>MDDKELIEYFKSQMKEDPDMASAVAAIRTLLEFLKRDKGETIQGLRANLTSAIETLCGVDSSVAVSSGGELFLRFISLASLEYSDYSKCKKIMIERGELFLRRISLSRNKIADLCHTFIKDGATILTHAYSRVVLRVLEAAVAAKKRFSVYVTESQPDLSGKKMAKALCHLNVPVTVVLDAAVGYIMEKADLVIVGAEGVVENGGIINKIGTNQMAVCAKAQNKPFYVVAESFKFVRLFPLNQQDVPDKFKYKADTLKVAQTGQDLKEEHPWVDYTAPSLITLLFTDLGVLTPSAVSDELIKLYL[2x];>[2x]MPGSDYKDHDGDYKDHDIDYKDDDDKAAKGSELSERIESFVETLKRGGGPRSSEEMARETLGLLRQIITDHRWSNAGELMELIRREGRRMTAAQPSETTVGNMVRRVLKIIREEYGRLHGRSDESDQQESLHKLLTSGGLNEDFSFHYAQLQSNIIEAINELLVELEGTMENIAAQALEHIHSNEVIMTIGFSRTVEAFLKEAARKRKFHVIVAECAPFCQGHEMAVNLSKAGIETTVMTDAAIFAVMSRVNKVIIGTKTILANGALRAVTGTHTLALAAKHHSTPLIVCAPMFKLSPQFPNEEDSFHKFVAPEEVLPFTEGDILEKVSVHCPVFDYVPPELITLFISNIGGNAPSYIYRLMSELYHPDDHVL;>MEFQAVVMAVGGGSRMTDLTSSIPKPLLPVGNKPLIWYPLNLLERVGFEEVIVVTTRDVQKALCAEFKMKMKPDIVCIPDDADMGTADSLRYIYPKLKTDVLVLSCDLITDVALHEVVDLFRAYDASLAMLMRKGQDSIEPVPGQKGKKKAVEQRDFIGVDSTGKRLLFMANEADLDEELVIKGSILQKHPRIRFHTGLVDAHLYCLKKYIVDFLMENGSITSIRSELIPYLVRKQFSSASSQQGQEEKEEDLKKKELKSLDIYSFIKEANTLNLAPYDACWNACRGDRWEDLSRSQVRCYVHIMKEGLCSRVSTLGLYMEANRQVPKLLSALCPEEPPVHSSAQIVSKHLVGVDSLIGPETQIGEKSSIKRSVIGSSCLIKDRVTITNCLLMNSVTVEEGSNIQGSVICNNAVIEKGADIKDCLIGSGQRIEAKAKRVNEVIVGNDQLMEI[2x];>[2x]MAAVAVAVREDSGSGMKAELPPGPGAVGREMTKEEKLQLRKEKKQQKKKRKEEKGAEPETGSAVSAAQCQVGPTRELPESGIQLGTPREKVPAGRSKAELRAERRAKQEAERALKQARKGEQGGPPPKASPSTAGETPSGVKRLPEYPQVDDLLLRRLVKKPERQQVPTRKDYGSKVSLFSHLPQYSRQNSLTQFMSIPS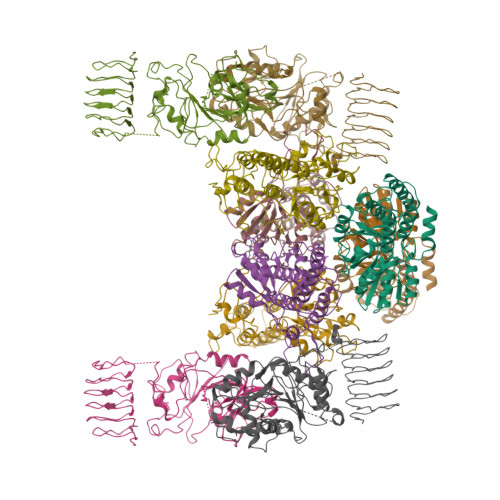SVIHPAMVRLGLQYSQGLVSGSNARCIALLRALQQVIQDYTTPPNEELSRDLVNKLKPYMSFLTQCRPLSASMHNAIKFLNKEITSVGSSKREEEAKSELRAAIDRYVQEKIVLAAQAISRFAYQKISNGDVILVYGCSSLVSRILQEAWTEGRRFRVVVVDSRPWLEGRHTLRSLVHAGVPASYLLIPAASYVLPEVSKVLLGAHALLANGSVMSRVGTAQLALVARAHNVPVLVCCETYKFCERVQTDAFVSNELDDPDDLQCKRGEHVALANWQNHASLRLLNLVYDVTPPELVDLVITELGMIPCSSVPVVLRVKSSDQ;>MAAPVVAPPGVVVSRANKRSGAGPGGSGGGGARGAEEEPPPPLQAVLVADSFDRRFFPISKDQPRVLLPLANVALIDYTLEFLTATGVQETFVFCCWKAAQIKEHLLKSKWCRPTSLNVVRIITSELYRSLGDVLRDVDAKALVRSDFLLVYGDVISNINITRALEEHRLRRKLEKNVSVMTMIFKESSPSHPTRCHEDNVVVAVDSTTNRVLHFQKTQGLRRFAFPLSLFQGSSDGVEVRYDLLDCHISICSPQVAQLFTDNFDYQTRDDFVRGLLVNEEILGNQIHMHVTAKEYGARVSNLHMYSAVCADVIRRWVYPLTPEANFTDSTTQSCTHSRHNIYRGPEVSLGHGSILEENVLLGSGTVIGSNCFITNSVIGPGCHIGDNVVLDQTYLWQGVRVAAGAQIHQSLLCDNAEVKERVTLKPRSVLTSQVVVGPNITLPEGSVISLHPPDAEEDEDDGEFSDDSGADQEKDKVKMKGYNPAEVGAAGKGYLWKAAGMNMEEEEELQQNLWGLKINMEEESESESEQSMDSEEPDSRGGSPQMDDIKVFQNEVLGTLQRGKEENISCDNLVLEINSLKYAYNISLKEVMQVLSHVVLEFPLQQMDSPLDSSRYCALLLPLLKAWSPVFRNYIKRAADHLEALAAIEDFFLEHEALGISMAKVLMAFYQLEILAEETILSWFSQRDTTDKGQQLRKNQQLQRFIQWLKEAEEESSEDD[2x]> MVPISPIETVPVKLKPGMDGPKVKQWPLTEEKIKALVEICTEMEKEGKISKIGPENPYNTPVFAIKKKDSTKWRKLVDFRELNKRTQDFWEVQLGIPHPAGLKKKKSVTVLDVGDAYFSVPLDEDFRKYTAFTIPSINNETPGIRYQYNVLPQGWKGSPAIFQSSMTKILEPFAAQNPDIVIIQYMDDLYVGSDLEIGQHRTKIEELRQHLLRWGLTTPDKKHQKEPPFLWMGYELHPDKWTVQPIVLPEKDSWTVNDIQKLVGKLNWASQIYPGIKVRQLSKLLRGTKALTEVIPLTEEAELELAENREILKEPVHGVYYDPSKDLIAEIQKQGQGQWTYQIYQEPFKNLKTGKYARMRGAHTNDVKQLTEAVQKITTESIVIWGKTPKFKLPIQKETWETWWTEYWQATWIPEWEFVNTPPLVKLWYQLEKEPIVGAETFYVDGAANRETKLGKAGYVTNKGRQKVVPLTNTTNQKTELQA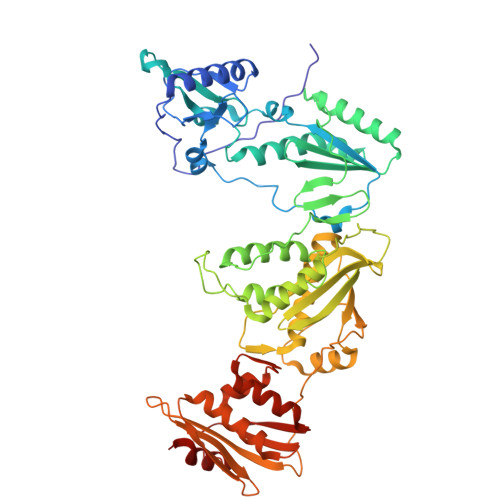IYLALQDSGLEVNIVTDSQYALGIIQAQPDKSESELVNQIIEQLIKKEKVYLAWVPAHKGIGGNEQVDKLVSAG> SNAMDRVATARAYYRALDEHDYDLLSDVLAPDFVHDRPDRTIEGRERFVRFMREERPQTDTSHPIATIYTGASTVAVEGRLLNS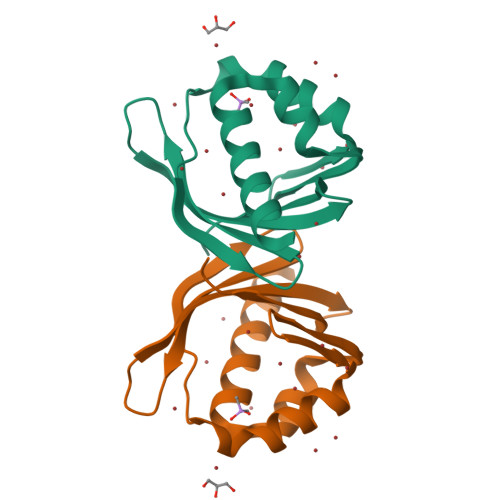DGAEITQFVDVFAFEDGVIGRIRTHTPEP> MGAEHLLEIFYLLLAAQVCAFIFKRLNQPVVIGEVLAGVLVGPALLGLVHEGEILEFLAELGAVFLLFMVGLETRLKDILAVGKEAFLVAVLGVALPFLGGYLYGLEIGFETLPALFLGTALVATSVGITARVLQELGVLSRPYSRIILGAAVIDDVLGLIVLACVNGVAETGQVEVGAITRLIVLSVVFVGLAVFLSTLIARLPLERLPVGSPLGFALALGVGMAALAASIGLAPIVGAFLGGMLLSEVREKYRLEEPIFAIESFLAPIFFAMVGVRL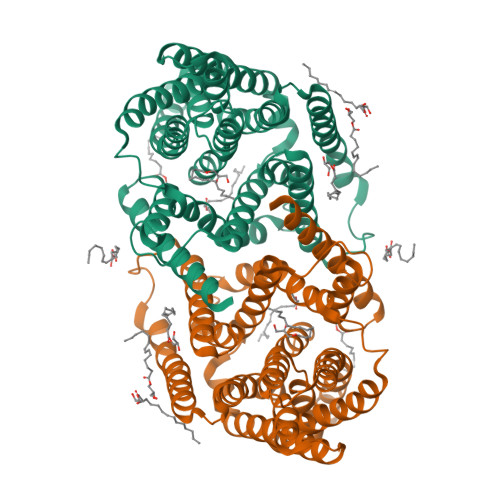ELSALASPVVLVAGTVVTVIAILGKVLGGFLGALTQGVRSALTVGCGMAPRGEVGLIVAALGLKAGAVNEEEYAIVLFMVVFTTLFAPFALKPLIAWTERERAAKE>[2x]GPMGSVSSGQAHSLTSLAKTWAARGSRSREPSPKTEDNEGVLLTEKLKPVDAEYREEVHWATHQLRLGRGSFGEVHRMEDKQTGFQCAVKKVSLEVFRAEELMACAGLTSPRIVPLYGAVREGPAVNIFMELLEGGSLGQLVKEQGCLPEDRALYYLGQALEGLEYLHSRRILHGDVKADNVLLSSDGSHAALCDFGHAVCLQPDGLGKSLLTGDYIPGTETHMAPEVVLGRSC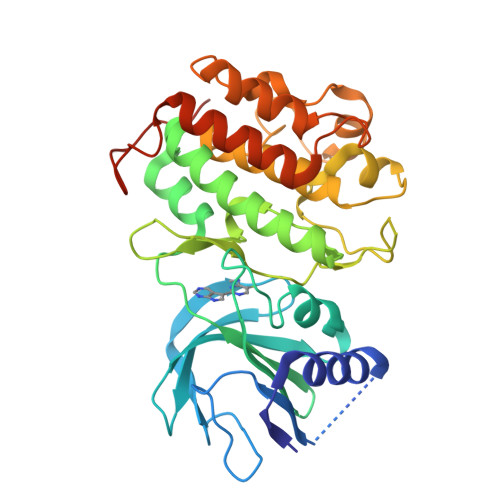DAKVDVWSSCCMMLHMLNGCHPWTQFFRGPLCLKIASEPPPVREIPPSCAPLTAQAIQEGLRKEPIHRVSAAELGGKVNRALQQVGGLKSPWRGEYKEPRHPPPNQANYHQTL>HMSLVTTSTSDGICTVKINRPDKLNAMNTDVAKELIKTFEELNHNDDVKVIILTGEGEKAFSAGADIEYMSKISADESVEYAKTGQLVTATVELVKQPTIAAVNGFALGGGCELAMSCDIRIAADTAKLGQPEVTIGVPPGWGGTQRLMRIV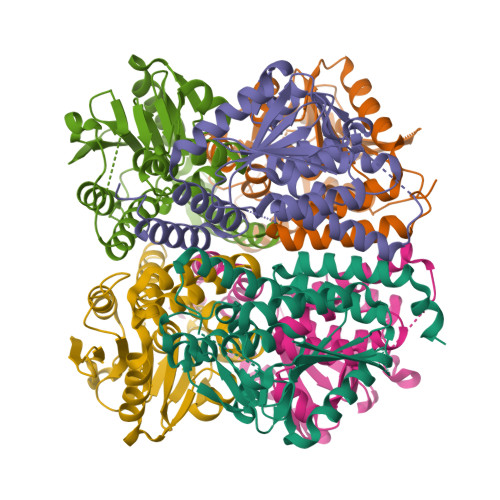GIAKAKELVYTGKMIKAEEAKEIGLVNHVVPLASLQEEALKMAQQIAGNSTMGVQMSKVAINKGRNADLDTGLGLEILAWRNCFTHPDRQERMTAFVNKSKK[6x]> MGPITPSTYVRCLNVGLIRKLSDFIDPQEGWKKLAVAIKKPSGDDRYNQFHIRRFEALLQTGKSPTSELLFD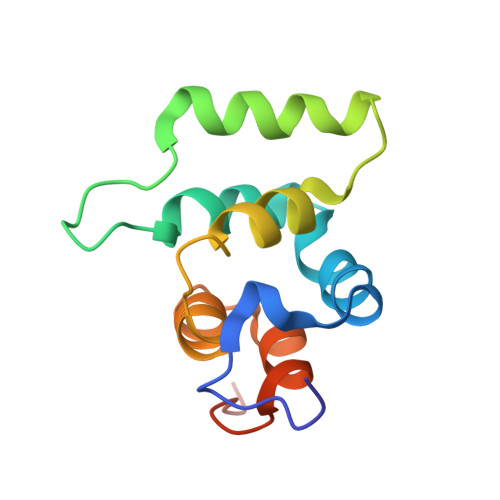WGTTNCTVGDLVDLLIQNEFFAPASLLLPDAVPLEHHHHHH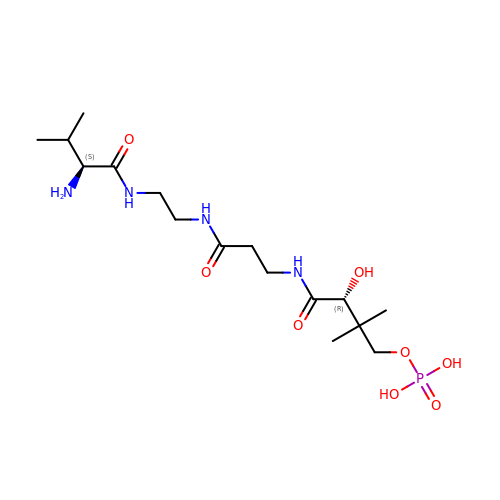[(3~{R})-4-[[3-[2-[[(2~{S})-2-azanyl-3-methyl-butanoyl]amino]ethylamino]-3-oxidanylidene-propyl]amino]-2,2-dimethyl-3-oxidanyl-4-oxidanylidene-butyl] dihydrogen phosphate | C16 H33 N4 O8 P | MFHZIFARQCIIMR-STQMWFEESA-N>[2x]GPLGSMGKKSRVKTQKSGTGATATVSPKEILNLTSELLQKCSSPAPGPGKEWEEYVQIRTLVEKIRKKQKGLSVTFDGKREDYFPDLMKWASENGASVEGFEMVNFKEEGFGLRATRDIKAEELFLWVPRKLLMTVESAKNSVLGPLYSQDRILQAMGNIALAFHLLCERASPNSFWQPYIQTLPSEYDTPLYFEEDEVRYLQSTQAIHDVFSQYKNTARQYAYFYKVIQTHPHANKLPLKDSFTYEDYRWAVSSVMTRQNQIPTEDGSRVTLALIPLWDMCNHTNGLITTGYNLEDDRCECVALQDFRAGEQIYIFYGTRSNAEFVIHSGFFFD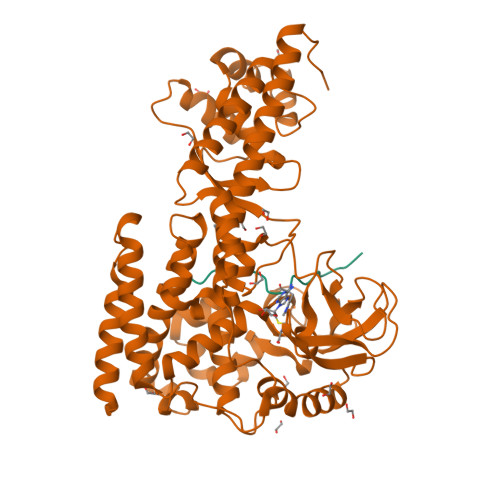NNSHDRVKIKLGVSKSDRLYAMKAEVLARAGIPTSSVFALHFTEPPISAQLLAFLRVFCMTEEELKEHLLGDSAIDRIFTLGNSEFPVSWDNEVKLWTFLEDRASLLLKTYKTTIEEDKSVLKNHDLSVRAKMAIKLRLGEKEILEKAVKSAAVNREYYRQQMEEKAPLPKYEESNLGLLESSVGDSRLPLVLRNLEEEAGVQDALNIREAISKAKATENGLVNGENSIPNGTRSENESLNQESKRAVEDAKGSSSDSTAGVKE;>[2x]TLKYPIEHGIVTNWD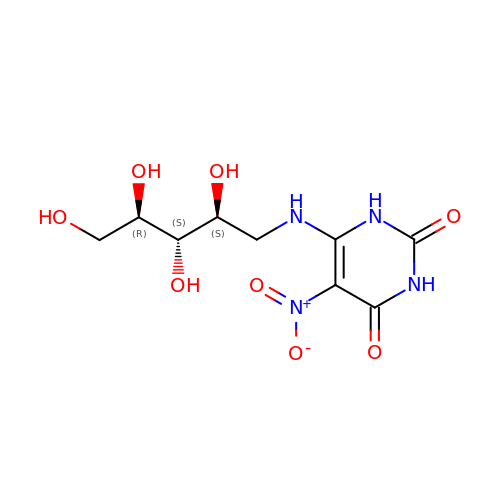5-NITRO-6-RIBITYL-AMINO-2,4(1H,3H)-PYRIMIDINEDIONE | C9 H14 N4 O8 | KSKGHNZSCSCHEQ-RPDRRWSUSA-N> GLPVYVTPGSGQFMTTDDMQSPCALPWYHPTKEIFIPGEVKNLIEMCQVDTLIPINSTQSNIGNVSMYTVTLSPQTKLAEEIFAIKVDIASHPLATTLIGEIASYFTHWTGSLRFSFMFCGTANTTLKVLLAYTPPGIGKPRSRKEAMLGTHVVWDVGLQSTVSLVVPWISASQYRFTT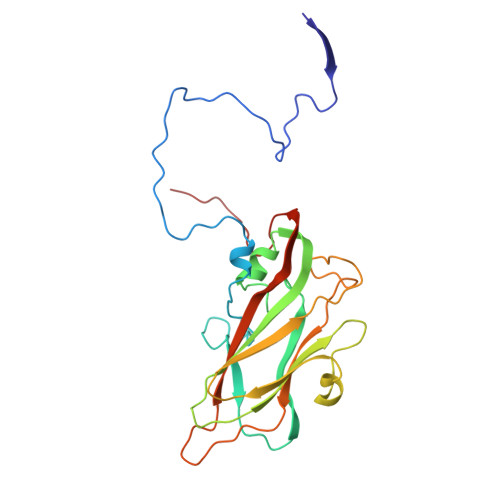PDTYSSAGYITCWYQTNFVVPPNTPNTAEMLCFVSGCKDFCLRMARDTDLHKQTGPITQ>SMKKYKLSEIHHLHPEYVRVSEHFKASMKNFKIEKIKKIENSELLDKFTWKKSQMKEEGKLLFYATSRAYVESICSNNFDSFLHETNENKYGKGIYFAKDAIYSHKYCPYDAKNVVMFVAQVLVGKFIEGNI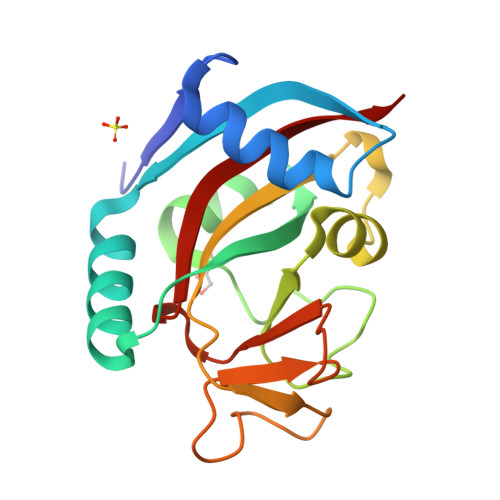TYTSPPPQFDSCVDTRSNPSVFVIFQKDQVYPQYVIEYTED[4x]> MSLSGTLIGAAAGGTVGLVASIYRDSKRKIIRDLQKQDIQYVEYGDTRTLIIPTDKYFMFSSPRLNEICYPGLNNVIRLLNFYPQSTIYVAGFTDNVGSRSHKRKLSQAQAETMMTFLWANGIAAKRLKAEGYGDKNAISDNAIIHGSAQNRRIEIQWFTSE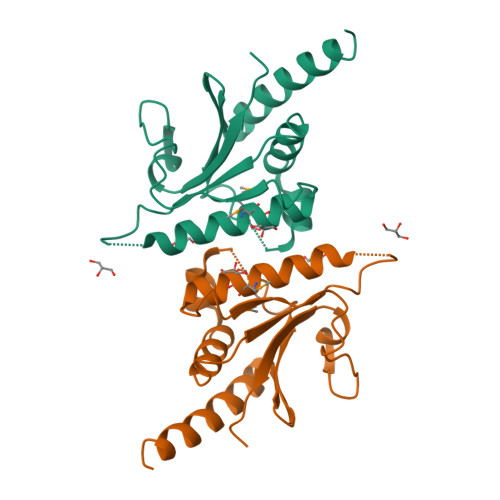GHHHHHH> MRLFVSDGVPGCLPVLAAAGRARGRAEVLISTVGPQDCVVPFLTRPKVPVL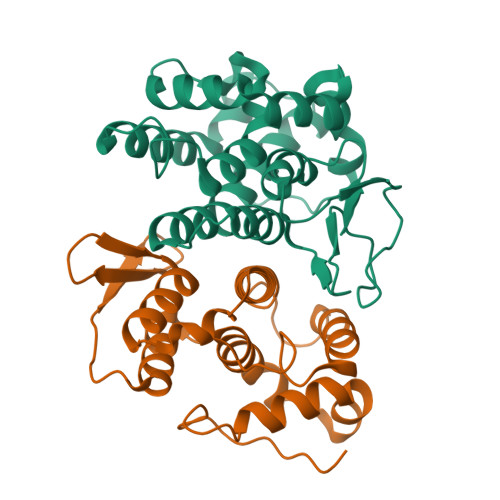QLDSGNYLFSTSAICRYFFLLSGWEQDDLTNQWLEWEATELQPALSAALYYLVVQGKKGEDVLGSVRRALTHIDHSLSRQNCPFLAGETESLADIVLWGALYPLLQDPAYLPEELSALHSWFQTLSTQEPCQRAAQTVLKQQGVLALRPYLQKQPQPSPAEGRAVTNEPEEEELEHHHHHH;> MRGSHHHHHHGSMAAAAELSLLEKSLGLSKGNKYSAQGERQIPVLQTNDGPSLTGLTTIAAHLVKQANKEYLLGSTAEEKAIVQQWLEYRVTQVDGHSSKNDIHTLLKDLNSYLEDKVYLTGYNFTLADILLYYGLHRFIVDLTVQEKEKYLNVSRWFSHIQHYPGIRQHLSSVVFIKNRLYTNSH>[2x]GSYQLEKEPIVGAETFYVDGAANRETKLGKAGYVTNKGRQKVVPLTNTTNQKTELQAIYLALQDSGLEVNIVTDSQY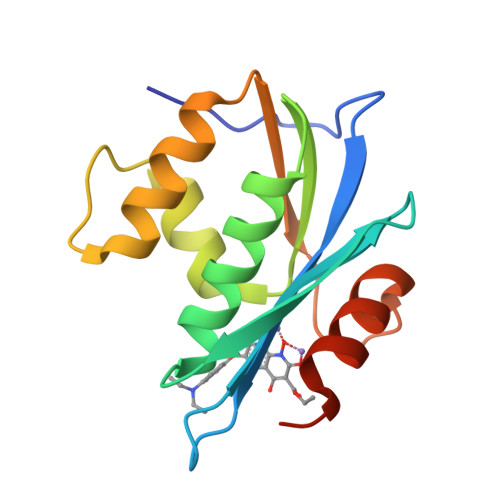ALGIIQAQPDKSESELVNQIIEQLIKKEKVYLAWVPAHKGIGGNEQVDKLVSAGIRKILFL Protein kinase D is a serine-threonine kinase comprising two N-terminal C1 domains, a PH domain and a C-terminal kinase domain belonging to the Ca2+/calmodulin-dependent kinase (CAMK) family. PKD signaling is tightly controlled by the lipid second messenger diacylglycerol (DAG), which in cells is produced by phospholipase C (PLC) downstream of either GPCR or receptor tyrosine kinase signaling. DAG recruits PKD via its two C1 domains to specific membranes in the cell, such as the plasma membrane and the TGN, where PKD is reportedly active. A second requirement for PKD activation is the phosphorylation of two serine residues (Ser738 and Ser742 in human PKD1) in the activation loop of the kinase domain.

To determine the structure of this module, a construct comprising the N-terminal and C1a domain of the C. elegans PKD homolog DKF-1 was purified and crystallized. Crystals diffracted to 2.2 Å, and the structure could be solved by experimental single anomalous dispersion phasing using the anomalous scattering of the Zn2+ ions in the C1a domain. The crystal structure reveals a dimeric assembly of the protein, in which the dimer interface sits on a crystallographic axis. Dimerization is mediated by the N-terminal domain, which adopts a ubiquitin-like fold. The dimerization interface on the ULD is mostly composed of hydrophobic residues. Using the structure of the isolated ULD dimer (residues 12–98) and the PDBePISA server, an interface area of 751 Å2 and a solvation free energy (ΔG) of −5.4 kcal/mol were calculated for the dimerization interface. To validate the dimerization interface observed in the crystal structure, we mutated the central hydrophobic phenylalanine to a negatively charged glutamate (F59E), the rationale being that two negatively charged residues in the interface should repel each other. Indeed, the F59E mutation converted the ULD and ULD–C1a into exclusive monomers. Aside from ULD dimerization, the structure also revealed an intramolecular interaction between the ULD and its corresponding C1a domain. This interface, in combination with the dimerization interface, gives rise to a unique arrangement of the C1 domains, with their respective DAG binding sites pointing in almost exactly opposite directions and contains three highly conserved residues in the ULD, Arg17, Arg22, and Glu85, that form a contiguous surface on the domain outside of the dimer interface.

> GAMDGSQGSTDYGDHVVLRYGGTREMVPLIRHEQMLDMLMERARQIVQGFGNLDTRNMYLFRHEYNSPTLLYPITSASQITSGSILEIILVDRTEAAVIPHVVEPESYMRPTFCDFCGEMLTGLMRQGVKCKNCNGNFHKRCSNAARNNCGAP>MEAHNQFLKTFQKERHDMKEAEKDEILLMENSRRFVMFPIKYHEIWAAYKKVEASFWTAEEIELAKDTEDFQKLTDDQKTYIGNLLALSISSDNLVNKYLIENFSAQLQNPEGKSFYGFQIMMENIYSEVYSMMVDAFFKDPKNIPLFKEIANLPEVKHKAAFIERWISNDDSLYAERLVAFAAKEGIFQAGNYASMFWLTDKKIMPGLAMANRNICRDRGAYTDFSCLLFAHLRTKPNPKIIEKIITEAVEIEKEYYS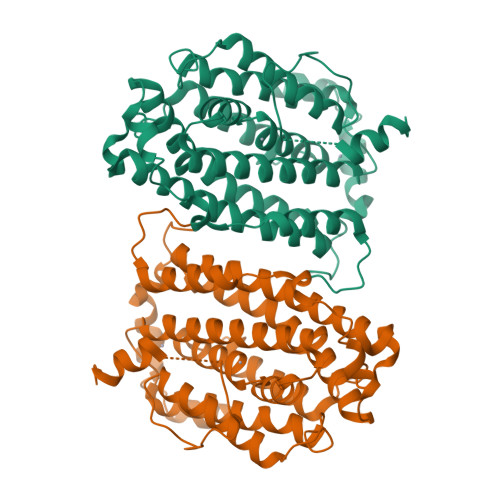NSLPVEKFGMDLKSIHTYIEFVADGLLQGFGNEKYYNAVNPFEFMEDVATAGKTTFFEKKVSDYQKASDMSKSATPSKEINFDDDF[2x]>[6x]MQKEEQDFLSPHVMLGYPESLDEQEEGERELREVQRIWSSAVPFNDLPEDEAQLIKTMFQITKVSNATLKKFGVRLFKPTKSLVFPWFAGPDSSLKGLKLLSAQNTDTEKVTYNEATVPKISSYYNLFGLTLVGRMDSEVVLTGHELDTLAVSQATGLPSVALPRGVSCLPPMLLPYLEQFKRVTLWLGHDIRSWEASKIFSRKLGLRRCSLVRPGEDRPCPLEALARGKNLSRIIKTSIPAAHKSIVSFKQLREDVYGELLNTEQVAGVKWTRFPELNRILKGHRKGE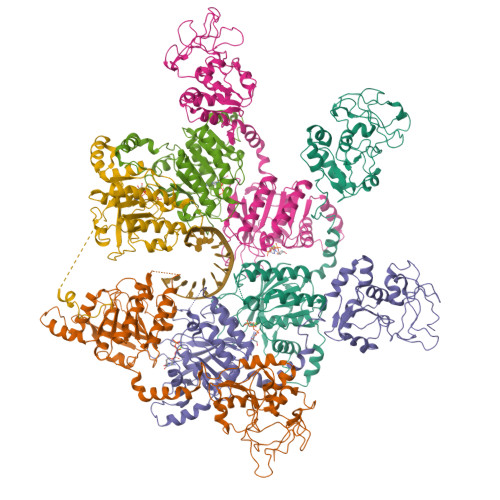LTVFTGPTGSGKTTFISEVALDLCIQGVNTLWGSFQINNVRLAKIMLTQFAMQRLEENLEQYDFWADKFEELPLYFMTFHGQQNIKTVLDTMQHAVYLYDINHVIIDNLQFMMGQENLSIDKYAVQDHIIGAFRKFATNTSCHVTLIIHPRKEEDDRELQTASIFGSAKASQEADNVLILQEKKLVTCPGRRSLQVTKNRFDGDVGIFPLDFIKSSLTFSAPIKGKVKLRKVSTKPENEEVGGERGGSEEGRG>MVVLAGPPAVDHIPLLRSPDPGDVFSGVPVVDLGSPGAARAVVDACERYGFFKVVNHGVATDTMDKAESEAVRFFSQTQPDKDRSGPAYPFGYGSKRIGFNGDMGWLEYLLLALDDASLADACTVPSCAVFRAALNEYISGVRKVAVRVMEAMSEGLGIAQADALSALVTAEGSDQVFRVNHYPPCRALQGLGCSVTGFGEHTDPQLVSVLRSNGTSGLQIALRDGQWVSVPSDRDSFFVNVGDSLQVLTNGRFKSVKHRVVANSLKSRVSFIYFGGPPLAQRIAPLPQLLGEGEQSLYKEFTWDEYKKAAYKSRLGDNRLAQFEKK[4x]

Here, we determined an X-ray crystal structure and performed functional analyses of two rice 2ODD family enzymes, OsGA2ox3 and OsDAO, which catabolize plant growth hormones GA4 and IAA, respectively. Both enzymes formed tetramers for OsGA2ox3, and dimers for OsDAO with the aid of their substrates, thereby enhancing their activity, as schematically summarized in Fig. 5c. With increasing substrate concentration, the enzyme gradually forms a multimer with the aid of the substrate itself (effecter), thereby resulting in an increase in enzymatic activity and in the active catabolism of GA or IAA to maintain hormonal homeostasis. The results revealed that a monomer–multimer switching occurs based on a substrate level, and that the resulting conformational change enhances the activities of these enzymes to maintain phytohormone homeostasis, in full agreement with the allosteric theory by Monod and co-workers.

GA 2-oxidase 3 (GA2ox3) is a member of the 2-oxoglutarate (2OG)- and Fe (II)-dependent dioxygenase (2ODD) enzyme family that requires 2OG and molecular oxygen as co-substrates, and ferrous iron Fe(II) as a co-factor, to inactivate biologically active GA4. We crystallized the enzyme with the co-substrates, 2OG and GA4 in the absence Fe(II) to prevent its enzymatic action and determined its structure via X-ray crystallography at a resolution of 2.15 Å. The crystallized protein consisted of a homotetramer (see below), whose each subunits with a common core fold in 2ODD enzyme family. As the location of amino acid residues in OsGA2ox3 interacting with Fe(II) are the same as that reported for other 2ODD enzymes, and Fe(II) was absent from crystalized OsGA2ox3, we located Fe(II) at the same position. While GA4 interacted with non-conserved amino acids, such as Q206, Y312, Y89, Y109, and R179, among 2ODD enzymes (green characters in Fig. 2b and green closed triangle in Supplementary Fig. 3). Additionally, GA4 also interacted with 2OG located at the bottom of the active-site cavity. K313 in subunit A directly interacted with P87 and F91 in subunit D by a hydrogen bond, and vice versa. In contrast, peak T corresponding to the tetramer appeared in the presence of GA4 (GA2ox3 + GA4), confirming that tetramerization was induced by the presence of GA4.> MENVVSAPMPGKVLRVLVRVGDRVRVGQGLLVL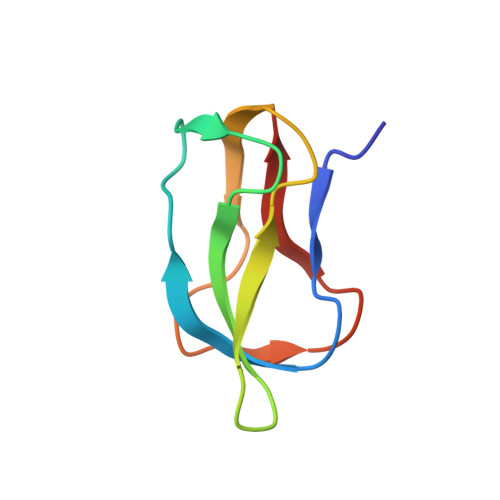EAMKMENEIPSPRDGVVKRILVKEGEIVDTGQPLIELG> GVGISTGTFNNQTEFKFLENGWVEITANSSRLVHLNMPESENYKRVVVNNMDKTAVKGNMALDDIHVEIVTPWSLVDANAWGVWFNPGDWQLI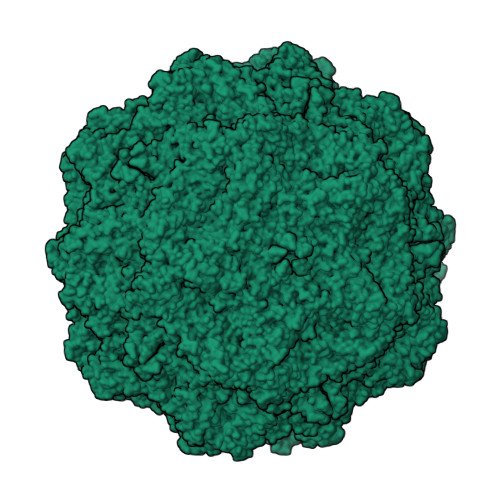VNTMSELHLVSFEQEIFNVVLKTVSESATQPPTKVYNNDLTASLMVALDSNNTMPFTPAAMRSETLGFYPWKPTIPTPWRYYFQWDRTLIPSHTGTSGTPTNVYHGTDPDDVQFYTIENSVPVHLLRTGDEFATGTFFFDCKPCRLTHTWQTNRALGLPPFLNSLPQSEGATNFGDIGVQQDKRRGVTQMGNTDYITEATIMRPAEVGYSAPYYSFEASTQGPFKTPIAAGRGGAQTDENQAADGDPRYAFGRQHGQKTTTTGETPERFTYIAHQDTGRYPEGDWIQNINFNLPVTNDNVLLPTDPIGGKTGINYTNIFNTYGPLTALNNVPPVYPNGQIWDKEFDTDLKPRLHINAPFVCQNNCPGQLFVKVAPNLTNQYDPDASANMSRIVTYSDFWWKGKLVFKAKLRASHTWNPIQQMSINVDNQFNYVPNNIGAMKIVYEKSQLAPRKLY4-[2-(5,5,8,8-TETRAMETHYL-5,6,7,8-TETRAHYDRO-NAPHTHALEN-2-YL)-[1,3]DIOXOLAN-2-YL]-BENZOIC 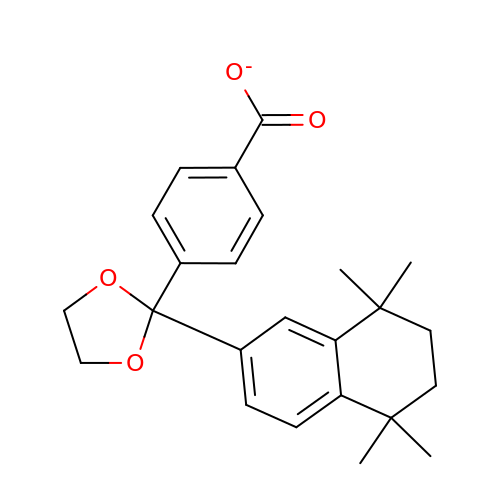ACID | C24 H27 O4 | ZZUKALQMHNSWTK-UHFFFAOYSA-M> MADTQYILPNDIGVSSLDSREAFRLLSPTERLYAYHLSRAAWYGGLAVLLQTSPEAPYIYALLSRLFRAQDPDQLRQHALAEGLTEEEYQAFLVYAAGVYSNMGNYKSFGDTKFVPNLPKEKLERVILGSEAAQQHPEEVRGLWQTCGELMFSLEPRLRHLGLGKEGITTYFSGNCTMEDAKLAQDFLDSQNLSAYNTRLFKEVDGCGKPYYEVRLASVLGSEPSLDSEVTSKLKSYEFRGSPFQVTRGDYAPILQKVVEQLEKAKAYAANSHQGQMLAQYIESFTQGSIEAHKRGSRFWIQDKGPIVESYIGFIESYRDPFGSRGEFEGFVAVVNKAMSAKFERLVASAEQLLKELPWPPTFEKDKFLTPDFTSLDVLTFAGSGIPAGINIPNYDDLRQTEGFKNVSLGNVLAVAYATQREKLTFLEEDDKDLYILWKGPSFDVQVGLHALLGHGSGKLFVQDEKGAFNFDQETVINPETGEQIQSWYRCGETWDSKFSTIASSYEECRAESVGLYLSLHPQVLEIFGFEGADAEDVIYVNWLNMVRAGLLALEFYTPEAFNWRQAHMQARFVILRVLLEAGEGLVTITPTTGSDGRPDARVRLDRSKIRSVGKPALERFLRRLQVLKSTGDVAGGRALYEGYATVTDAPPESFLTLRDTVLLRKESRKLIVQPNTRLEGSDVQLLEYEASAAGLIRSFSERFPEDGPEL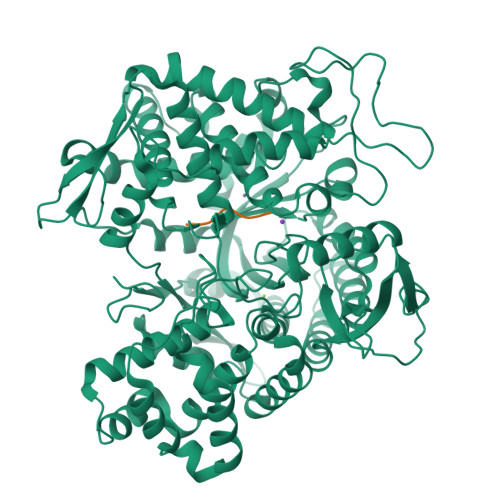EEILTQLATADARFW;> IVYPW> MTTYLEFIQQNEERDGVRFSWNVWPSSRLEATRMVVPVAALFTPLKERPDLPPIQYEPVLCSRTTCRAVLNPLCQVDYRAKLWACNFCYQRNQFPPSYAGISELNQPAELLPQFSSIEYVVLRGPQMPLIFLYVVDTCMEDEDLQALKESMQMSLSLLPPTALVGLITFGRMVQVHELGCEGISKSYVFRGTKDLSAKQLQEMLGLSKVPLTQATRGPQVQQPPPSNRFLQPVQKIDMNLTDLLGELQRDPWPVPQGKRPLRSSGVALSIAVGLLECTFPNTGARIMMFIGGPATQGPGMVVGDELKTPIRSWHDIDKDNAKYVKKGTKHFEALANRAATTGHVIDIYACALDQTGLLEMKCCPNLTGGYMVMGDSFNTSLFKQTFQRVFTKDMHGQFKMGFGGTLEIKTSREIKISGAIGPCVSLNSKGPCVSENEIGTGGTCQWKICGLSPTTTLAIYFEVVNQHNAPIPQGGRGAIQFVTQYQHSSGQRRIRVTTIARNWADAQTQIQNIAASFDQEAAAILMARLAIYRAETEEGPDVLRWLDRQLIRLCQKFGEYHKDDPSSF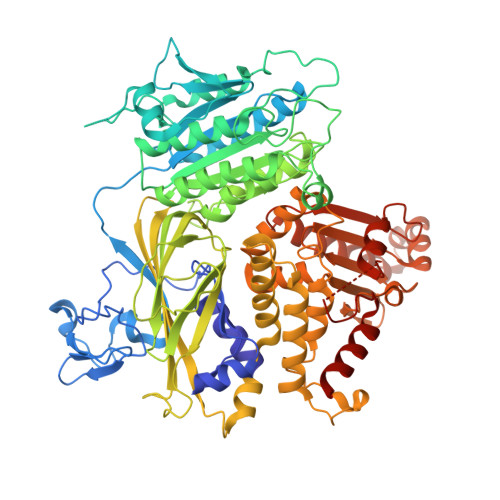RFSETFSLYPQFMFHLRRSSFLQVFNNSPDESSYYRHHFMRQDLTQSLIMIQPILYAYSFSGPPEPVLLDSSSILADRILLMDTFFQILIYHGETIAQWRKSGYQDMPEYENFRHLLQAPVDDAQEILHSRFPMPRYIDTEHGGSQARFLLSKVNPSQTHNNMYAWGQESGAPILTDDVSLQVFMDHLKKLAVSSAA We report the biochemical, structural, and functional characterization of the protein coded by gene PA4880 in the P. aeruginosa PAO1 genome. Our structural work shows that the product of gene PA4880 is a protein that adopts the Dps subunit fold, which oligomerizes into a 12-mer quaternary structure. Unlike Dps, however, the ferroxidase di-iron centers and iron coordinating ligands are buried within each subunit, in a manner identical to that observed in the ferroxidase center of P. aeruginosa bacterioferritin. The ferroxidase centers in Pa DpsL catalyze the oxidation of Fe2+ utilizing O2 or H2O2 as oxidant, and the resultant Fe3+ is compartmentalized in the interior cavity.

Prismatic crystals were also obtained from the Salt RxHT screen condition G2 (1 M MgSO4, 100 mM Bis-Tris pH 7.0). Structure solution and refinement produced the model termed Pa DpsL-dd-Mg (3.0 Å resolution), which contains 44 sulfate ions, 24 Fe ions, and 37 Mg ions. The locations of the Mg2+ ions were identified by analyzing the Fo-Fc difference electron density following refinement and by computing a Fo-Fo electron density difference map to compare the differences between the DpsL-dd-Mg and DpsL-dd data sets. Except for the presence of Mg2+, the structural features observed in the Pa DpsL-dd-Mg are nearly identical to those observed in the Pa DpsL-dd structure. A network of Mg2+ and SO4 2- ions are observed in the structures of 12-mer Pa DpsL (Pa DpsL-dd and Pa DpsL-dd-Mg). Four distinct SO4 2- and three unique Mg2+ binding sites have been observed. Both types of ions can be visualized in the Pa DpsL-dd-Mg structure The SO4 2- binding sites can be observed in sites 1–4. Two Mg2+ ions (Mg site 1) are in proximity to sulfate site 2, where each of the cations is coordinated by the side chain of Glu 106, which stems from each of the one-turn α3 helices. Mg site 2 is near the protein surface where it is coordinated by the side chains of Asp 167 and Asp 171 in the C-terminal helix (α5), whereas Mg site 3 is in the 12-mer interior, where it is coordinated by the side chains of Asp164, Asp168 in the C-terminal helix and Glu 72 and Glu75 in helix α2. This extensive network of Mg2+ and SO4 2- ions coordinated to 12-mer DpsL suggest that the nature of the stabilizing effect that Mg2+ and SO4 2- have on the DpsL dodecamer structure originate from the mediation of otherwise repulsive electrostatic interactions that would take place among positively charged residues in the three-fold pores, or among the high density of negative charge concentrated near the C-terminus. Hence, in the absence of Mg2+ and SO4 2-, one can envision significant folding-unfolding transitions affecting secondary, tertiary, and quaternary structure, which largely destabilize not only the 12-mer structure but also lead to proteolysis of the N-terminal domain.

>[12x]MTTVQLTDVQTLRDRARKNIQEGAVTEGYSADRQTVLRLLNEALATELVCFLRYKRHYFMATGLKASIAAAEFLEHANQEMQHADQLAERIMQLGGEPDFNPRGLEERSHAEYVEGKTLKDMVTENLIAERIAIDSYREIITYLGNDDPTTRRIFEEILAQEEEHADDMADILDDLA> VVQYLNQELVVSGKIDFENAEQQYQAGLAI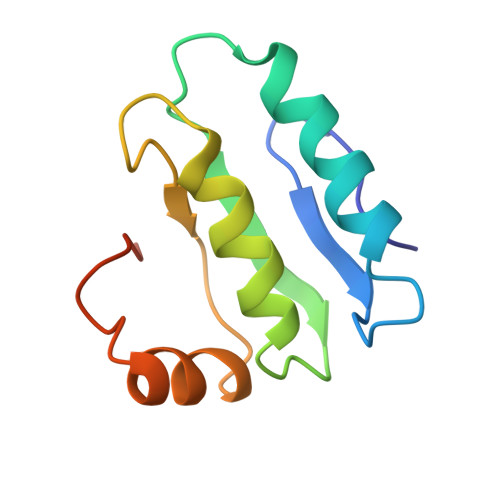IKKQTSFPLIVDLKQLEHGNTLALAVLVQWLRQTPQKSGLHFKNVPEKMLKIIQACHLQEDLHLVLEHHHHHH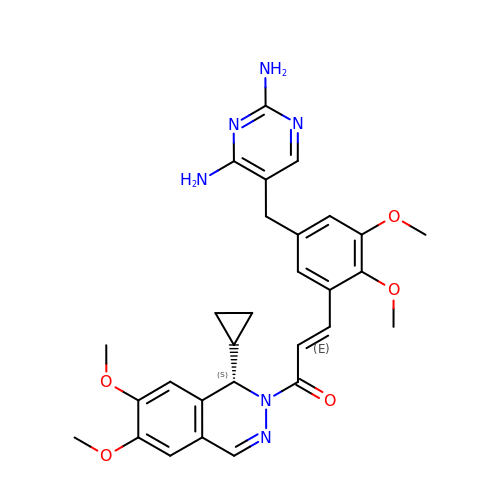(2E)-1-[(1S)-1-cyclopropyl-6,7-dimethoxy-3,4-dihydrophthalazin-2(1H)-yl]-3-{5-[(2,4-diaminopyrimidin-5-yl)methyl]-2,3-dimethoxyphenyl}prop-2-en-1-one | C29 H32 N6 O5 | WEOHMFQXNAIIAE-GJTXFRBNSA-N>[24x]MTEKTPDDVFKLAKDEKVEYVDVRFCDLPGIMQHFTIPASAFDKSVFDDGLAFDGSSIRGFQSIHESDMLLLPDPETARIDPFRAAKTLNINFFVHDPFTLEPYSRDPRNIARKAENYLISTGIADTAYFGAEAEFYIFDSVSFDSRANGSFYEVDAISGWWNTGAATEADGSPNRGYKVRHKGGYFPVAPNDQYVDLRDKMLTNLINSGFILEKGHHEVGSGGQAEINYQFNSLLHAADDMQLYKYII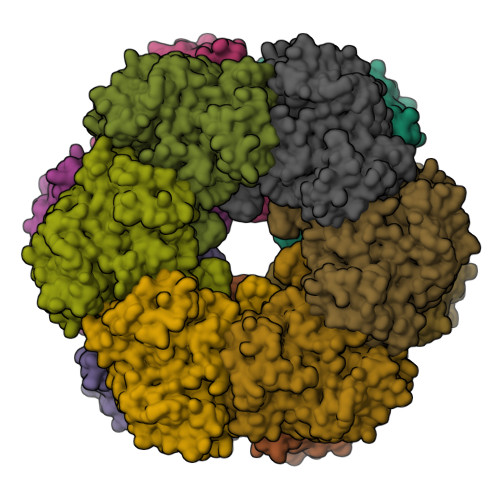KNTAWQNGKTVTFMPKPLFGDNGSGMHCHQSLWKDGAPLMYDETGYAGLSDTARHYIGGLLHHAPSLLAFTNPTVNSYKRLVPGYEAPINLVYSQRNRSACVRIPITGSNPKAKRLEFRSPDSSGNPYLAFSAMLMAGLDGIKNKIEPQAPVDKDLYELPPEEAASIPQTPTQLSDVIDRLEADHEYLTEGGVFTNDLIETWISFKRENEIEPVNIRPHPYEFALYYDV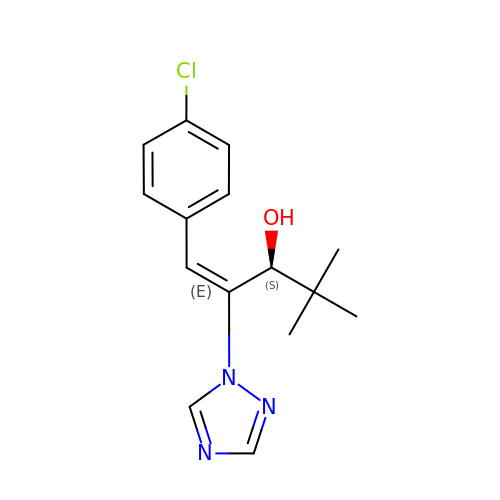(1E,3S)-1-(4-chlorophenyl)-4,4-dimethyl-2-(1H-1,2,4-triazol-1-yl)pent-1-en-3-ol | C15 H18 Cl N3 O | YNWVFADWVLCOPU-MAUPQMMJSA-N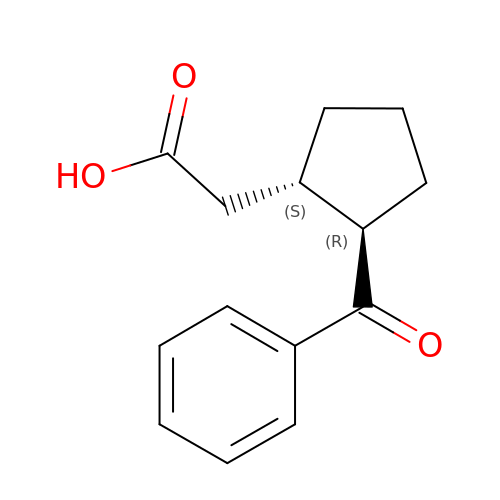[(1S,2R)-2-(benzenecarbonyl)cyclopentyl]acetic acid | C14 H16 O3 | NMNCOSWJMSHIOO-NWDGAFQWSA-N> MAEGEITTFTALTEKFNLPPGNYKKPKLLYCSNGGHFLRILPDGTVDGTRDRSDQHIQLQLSAESVGEVYIKSTETGQYLAMDTDGLLYGSQT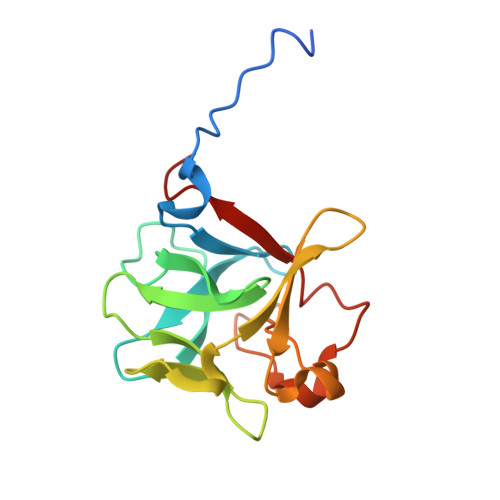PNEECLFLERLEENHYNTYISKKHAEKNWFVGLKKNGSCKRGPRTHYGQKAILFLPLPVSSD>[8x]GMSLANQIDQFLGTIMQFAENKHEILLGKCESDVKLTSTQEHILMLLAEQISTNAKIAEKLKISPAAVTKALKKLQEQELIKSSRATNDERVVLWSLTE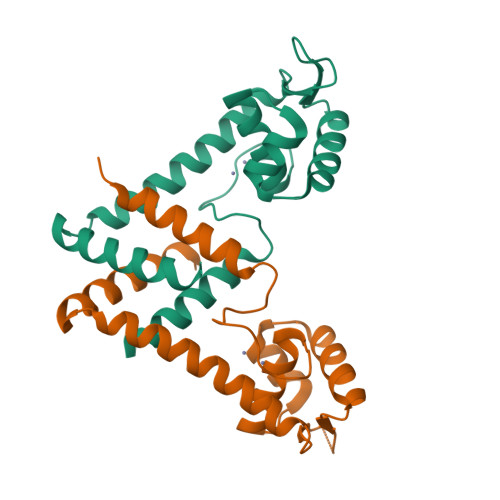KAVPVAKEHATHHEKTLSTYQELGNKFTDEEQEVISKFLSALTEEFQ> AGDNKGITYEELNPERFTLLEKGTPTNILIDENEDQGVMIAATNLSEDFGRVSGTNAPLIFLPDNERLIIVGTLESRYIKELTENRKIKGDELKGKNEKYLMTVVDNPLPGVKEALIIAGSDKRGAIYGIYELSEQIGVSPWYDWADVPVKPQQNLSIERGSYTADEPAVTYRGIFLNDEAPALTSWVENTYGTKYGDHRFYSRVFELILRLRGNFLWPAMWDWSFYGDDPLNSKTADTMGIIMGTSHHEPMARNHQEWARNRDKYGVWDYTSNQEVIDQFFREGIERVKDTDDLITIGMRGDGDTPMPMGVKEGEDHLPSDEDNMRLLERIIKNQREIIGDVTGESPEKTPQVWAIYKEVQRYFDLGLRPPEDVIILLSDDNWGNVRRLPTEEERDHPGGWGMYYHFDYVGAPRSSKWLNISPIQNIWEQMQLTYDYGVDELWVANVGDLKPMEYPITLFLDMAWDPTRFNAENLLDHTRSFAAQQFGEDQADEAARIINLYSKYNGRVTPEMLDRNTYNLESGEWKKVSDEYIKLEAEALRQYLTLEPEQRDAYKQLILYPVQAMANLYEMYYSQAMNHKLYRENNPMANYWADRVEETFNRDAELSHDYNKVMANGKWDGMMTQKKIGYRSWNDNFPADTLPQIFRIENPEEATGGYVFTARDGVVVIEAEHYFEAKD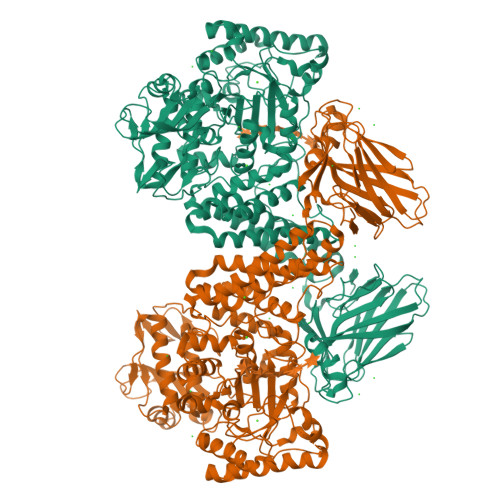AEEAKWTVIPYMGRTLSSIALMPYTKEVEGASLSYRMQIPDEVSEVKVHVVVKSTLPFHDPKGHEYRVGFEGGSKEIVNFNWNLNEEPENIYSVFYPTVASRVVKKDVTLDLHDTDDGFYTLTLEPLDPGIVFQKIVVDFGGYEESRLFMEESPNKRIEIE> QTGLDDSTMQSLKSSLNLTSDVDWSNPNPCKWQSVQCDGSNRVTKIQLKQKGIRGTLPTNLQSLSELVILELFLNRISGPIPDLSGLSRLQTLNLHDNLFTSVPKNLFSGMSSLQEMYLENNPFDPWVIPDTVKEATSLQNLTLSNCSIIGKIPDFFGSQSLPSLTNLKLSQNGLEGELPMSFAGTSIQSLFLNGQKLNGSISVLGNMTSLVEVSLQGNQFSGPIPDLSGLVSLRVFNVRENQLTGVVPQSLVSLSSLTTVNLTNNYLQGPTPLFGKSVGVDIV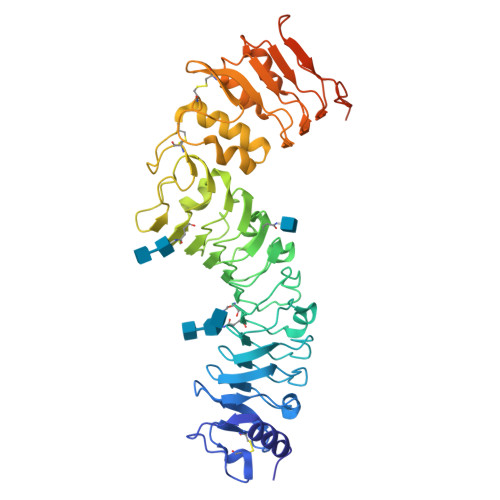NNMNSFCTNVAGEACDPRVDTLVSVAESFGYPVKLAESWKGNNPCVNWVGITCSGGNITVVNMRKQDLSGTISPSLAKLTSLETINLADNKLSGHIPDELTTLSKLRLLDVSNNDFYGIPPKFRDTVTLVTEGNANMGKNGPNKTSDAPGASPGSKPSGGSDGSETSKKSSNVK> HHHHHHHSSGLVP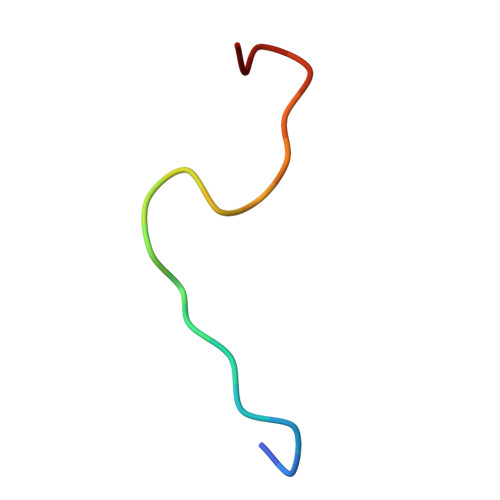RGSHA> MHLNPAEKEKLQIFLASELLLRRKARGLKLNYPEAVAIITSFIMEGARDGKTVAMLMEEGKHVLTRDDVMEGVPEMIDDIQAEATFPDGTKLVTVHNPIS;> MSNNNYIVPGEYRVAEGEIEINAGREKTTIRVSNTGDRPIQVGSHIHFVEVNKELLFDRAEGIGRRLNIPSGTAARFEPGEEMEVELTELGGNREVFGISDLTNGSVDNKELILQRAKELGYKGVE;> MKINRQQYAESYGPTVGDEVRLADTDLWIEVEKDYTTYGDEVNFGGGKVLREGMGENGTYTRTENVLDLLLTNALILDYTGIYKADIGVKDGYIVGIGKGGNPDIMDGVTPNMIVGTATEVIAAEGKIVTAGGIDTHVHFINPDQVDVALANGITTLFGGGTGPAEGSKATTVTPGPWNIEKMLKSTEGLPINVGILGKGHGSSIAPIMEQIDAGAAGLKIHEDWGATPASIDRSLTVADEADVQVAIHSDTLNEAGFLEDTLRAINGRVIHSFHVEGAGGGHAPDIMAMAGHPNVLPSSTNPTRPFTVNTIDEHLDMLMVCHHLKQNIPEDVAFADSRIRPETIAAEDILHDLGIISMMSTDALAMGRAGEMVLRTWQT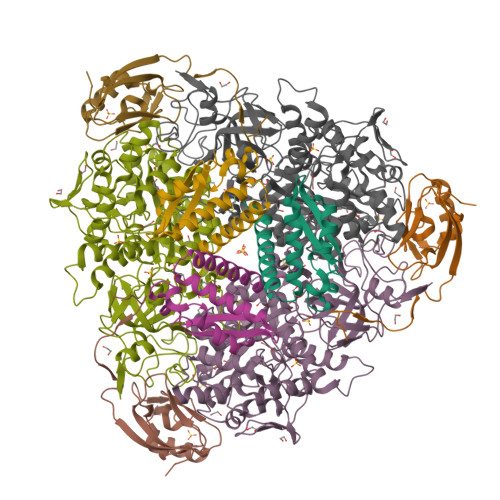ADKMKKQRGPLAEEKNGSDNFRLKRYVSKYTINPAIAQGIAHEVGSIEEGKFADLVLWEPKFFGVKADRVIKGGIIAYAQIGDPSASIPTPQPVMGRRMYGTVGDLIHDTNITFMSKSSIQQGVPAKLGLKRRIGTVKNCRNIGKKDMKWNDVTTDIDINPETYEVKVDGEVLTCEPVKELPMAQRYFLF> VSKKPSLSVQPGPIVAP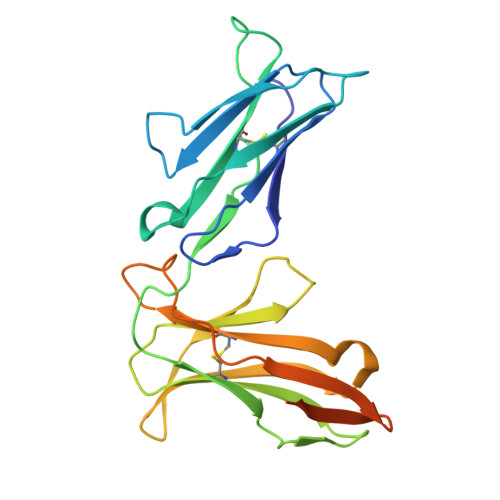EETLTLQCGSDAGYNRFVLYKDGERDFLQLAGAQPQAGLSQANFTLGPVSRSYGGQYRCYGAHNLSSEWSAPSDPLDILIAGQFYDRVSLSVQPGPTVASGENVTLLCQSQGWMQTFLLTKEGAADDPWRLRSTYQSQKYQAEFPMGPVTSAHAGTYRCYGSQSSKPYLLTHPSDPLELVVSGGGGLEVLFQGPGGSAWSHPQFEKGGHHHHHHHH>SPMAVEEVIEMQGLSLDPTSHRVMAGEEPLEMGPTEFKLLHFFMTHPERVYSREQLLNHVWGTNVYVEDRTVDVHIRRLRKALE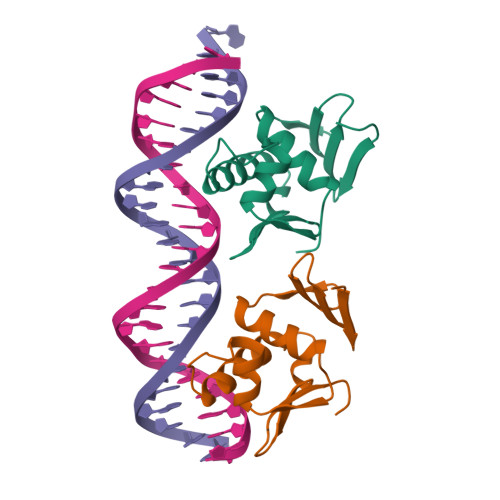PGGHDRMVQTVRGTGYRFSTRF[4x]> SIVTKSIVNADAEARYLSPGELDRIKSFVSSGEKRLRIAQILTDNRERIVKQAGDQLFQKRPDVVSPGGNAYGQEMTATCLRDL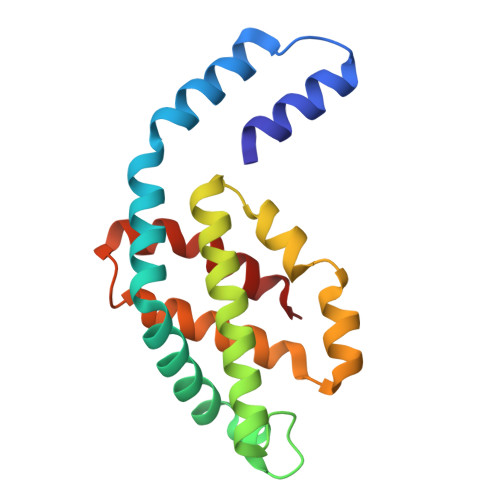DYYLRLITYGIVAGDVTPIEEIGIVGVREMYKSLGTPIDAVAAGVSAMKNVASSILSAEDAAEAGAYFDYVAGALA4-chloranyl-N-[[4-chloranyl-3-(3-chloranyl-5-cyano-phenoxy)-2-fluoranyl-phenyl]methyl]-1H-imidazole-5-carboxamide 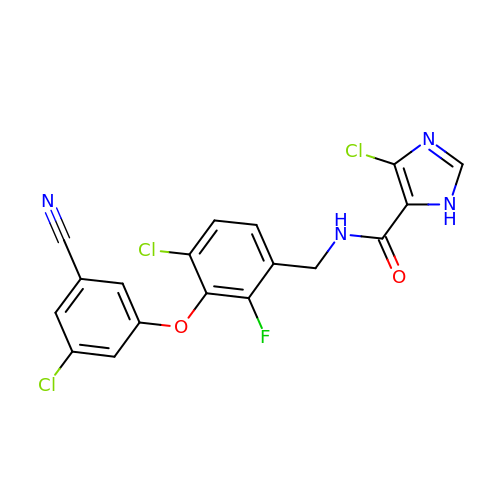| C18 H10 Cl3 F N4 O2 | FCSGFPSBYUHMIF-UHFFFAOYSA-N> MASADSRRLGDGDGAGGAFQPYLDSLRQELQQRDPTVLSVVVALLAVLLTLVFWKLVRSRRSSQRAVLLLGLCDSGKTLLFVRLLTGHYRDTQTSITDSSATYRVNNNRGNSLTLIDLPGHESLRLQFLERFKTSARAVVFVVDSAAFQREVKDVAEFLYQVLIDSMSLKNTPSFLIACNKQDIAMAKSAKLIQQQLEKELNTLRVTRSAAPSTLDSSSTAPAQLGKKGKEFEFSQLPLKVEFL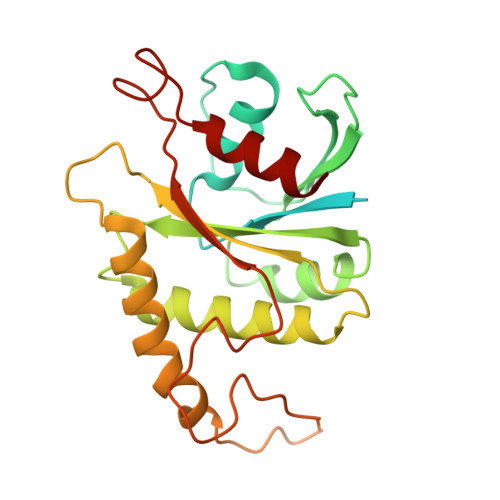ECSAKGGRGDPGSADIQDLEKWLAKIA In most bacteria, chromosome dimer resolution is performed by two site-specific recombinases, XerC and XerD, whereas in archaea only one such protein, XerA, is thought to play this role. The Xer enzymes belong to the tyrosine recombinase family (hereafter referred to as Tyr-recombinase) which is one of the two large classes of site-specific recombinases. Here we present the first crystal structure of a full-length archaeal Tyr-recombinase, the XerA recombinase from Pyrococcus abyssi. XerA displays the canonical two-domain structure of Tyr-recombinases and assembles as an apo-dimer.

Therefore the structure of full-length XerA was solved by molecular replacement in two stages, using the separate domains independently as search models. The final model has a resolution of 3.0 Å and displays good stereochemistry. Surprisingly, analysis of crystal packing of XerA revealed that two monomers, related by a crystallographic symmetry axis, form a putative dimer. The interactions in XerA are mainly stabilized by contacts between the two αK helices. The XerA structure revealed that the extreme C-terminal αN helix packs in cis into a groove located at the surface of the C-terminal domain. Within the XerA apo-dimer, positioning of the αN helix in cis prevents contacts between the αM helix and the catalytic site resulting in the exclusion of the catalytic Tyr from the active site. Interestingly, Y261 is located at the end of the most flexible loop of XerA, at the N-terminus of the αM helix, and is extruded away from the active site with its side chain pointing towards the solvent. The conserved catalytic residues R135 and H226 of XerA are within hydrogen-bonding distance of the sulfate ion. The simplest interpretation of these results is that XerA follows a cis cleavage mechanism despite the unusual orientation of the catalytic Tyr extruded from the XerA dimer.

> MEEREERVRDDTIEEFATYLELEGKSRNTVRMYTYYISKFFEEGHSPTARDALRFLAKLKRKGYSTRSLNLVIQALKAYFKFEGLDSEAEKLKTPKMPKTLPKSLTEEEVRRIINAAETLRDRLILLLLYGAGLRVSELCNLRVEDVNFEYGVIVVRGGKGGKDRVVPISESLLSEIKRYLESRNDDSPYLFVEMKRKRKDKLSPKTVWRLVKKYGRKAGVELTPHQLRHSFATHMLERGIDIRIIQELLGHSNLSTTQIYTKVSTKHLKEAVKKAKLVESIIGGSHHHHHH> MSRHQFDLIMCLKQPGVQTGLLCEKCDGKCPICDSYVRPKRKVRV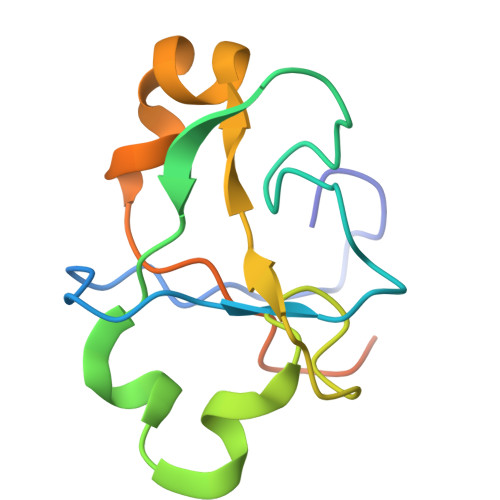CENCSFGKQAKNCIICNLNVGVNDAFYCWECCRLGKDKDGCPRILNLGSNRLDRHFEKKKKV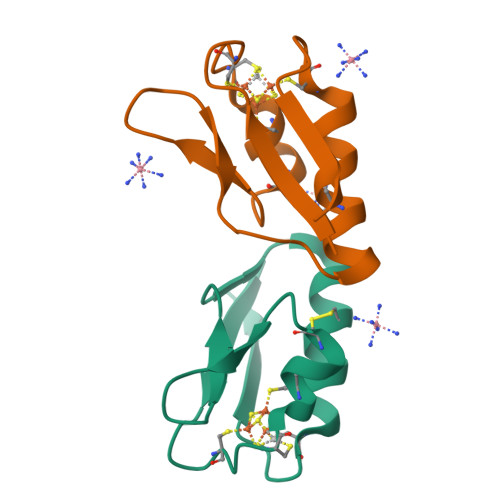>[2x]AWKVSVDQDTCIGCAICASLCPDVFEMNDEGKAQPKVEVIEDEELYNCAKEAMEACPVSAITIEEA>HHHHHHMQRKNDMQTQRLRIAIQKKGRLSQECQELLKKCGVKFNIMGERLVVHSLNMPIDLLLVRDDDIPGLIMDGVVDLGFVGENVLEETRLDRLALNQRNEFTTLRRMDFGGCRLSIAIEKDAEYRGPQDLNGKRIATTYPQLLKAYMDRQGVDFSTCMLTGSVEVAPRAGLADAIADLVSTGATLEANGLKEVEVIFE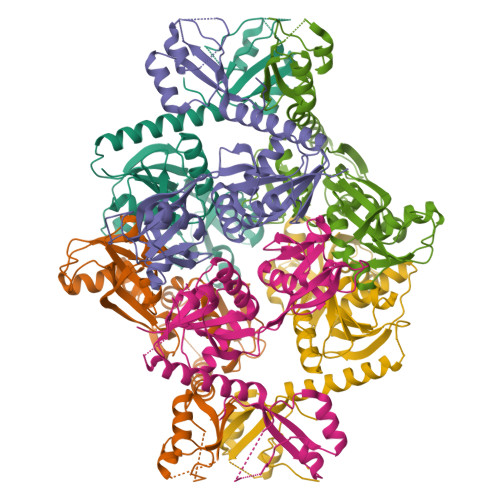SKATLIQRPGAFAADKAALIDKLLTRMHGVQQAKESKYIMLHAPVEKLAQIKTLLPGAEDPTVLPLSADKSKVAVHMVSSENLFWETMEQLKALGASSILVLPIEKMME[2x]> GKTITDFSISRSVLAKYEVINQVDKKFILIRCLDQSIHNCPLLVLVDQHACDERIRLEELFYSLLTEVVTGTFVARDLKDCCIEVDRTEADLFKHYQSEFKKWGIGYETIE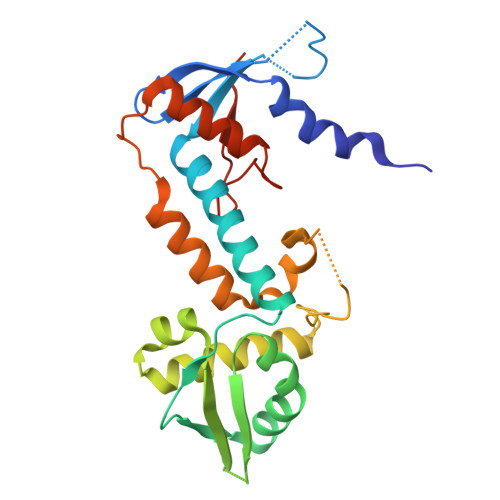GTMETSLLEIKTLPEMLTSKYNGDKDYLKMVLLQHAHDLKDFKKLPMDLSHFENYTSVDKLYWWKYSSCVPTVFHEILNSKACRSAVMFGDELTRQECIILISKLSRCHNPFECAHGRPSMVPIAEL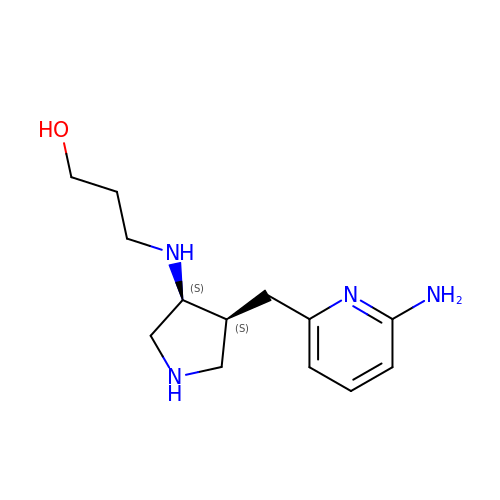3-({(3S,4S)-4-[(6-aminopyridin-2-yl)methyl]pyrrolidin-3-yl}amino)propan-1-ol | C13 H22 N4 O | SJAGNBCHAAJNEQ-CMPLNLGQSA-N> XXXXXXXX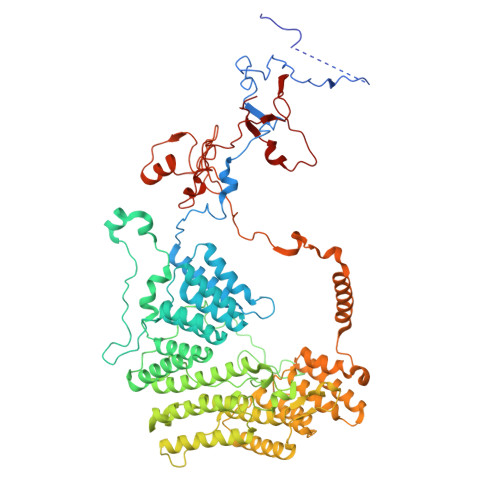XXXXXXXXXFVFRDPSLXXXXXXXXXXXXXXXXXXXXXXXXXXXXXXXHANTQYQHAWPLLSHDDLGNSDQSNNTKNIMYSMYMPKRNKGTAPWFRGADTYSVKYCEQGRYEYQRYLMINRFPSEYKKHFLSFLSNIRMSSGSATIPQEALHWLLRMIVDNFNPQHVHYIAAMKTLQSAGELDMARDVWKIMERQQTWPCTATICAYLDVCVEAGEKTWAMEAWNRYCTELKFLEPGEVDPKPISRVPFSLTREELLYLPKWKKHFDHDPNLDVMDLNRFNRTREVYLRMAQVMLAGGERNAFQHFFTKLEEAMLNKPTPVPEPPNPHLVRRPRWAPYEHCKSVHHSPWRLQNNGRALALGPPVTIEDEMQSRFFSNDQFLVHSVKEVLRIVLQEHKRAHPTECTRCKTEAFFYKTKDADETLKFCDDLIERLFASLGVRLSNLNTSSLLSTILEVFRVVGKESGAALLQRANEFLERKASLGDAEGSRENLTASNYLQVLSGFADESAFVYNTKKDGTCQYKTGFDPRTTMRHLADVVQEIAGNPHVTWAADMHLQVVETMVGCGTMKANDYFVRNVLRQFSWDSRFLEALYVEYRRQDDVDMWAELTKRALVWTARYNAPASERLRRLIEDDYDTIRVQTRTFRELAVFQFRDVEERRHSRDVVNELPNPWYDYVAHALPFPDRDAGYPDEYGDLGQWRAPGGPGSPVRGPGYYAPPMEGEHQRGYTAEWRDLRNPMRPPEFPTPWERKYRQYARGQHPSYDMVYAGPMPEIFPMRRDFRKPTRWDFHDIEKQGKYRTSGPY>GGGSMEPGRGGTETVGKFEFSRKDLIGHGAFAVVFKGRHRAAHDLEVAVKCINKKNLAKSQTLLGKEIKILKELKHENIVALYDFQEMANSVYLVMEYCNGGDLADYLHAMRTLSEDTIRLFLQQIAGAMRLLHSKGIIHRDLKPQNILLSNPAGRRANPNSIRVKIADFGFARYLQSNMMAATLCGSPMYMAPEVIMSQHYDGKADLWSIGTIVYQCLTGKAPFQASSPQDLRLFYEKNKTLVPTIPRETSAPLRQLLLALLQRNHKDRMDFDEFFHHP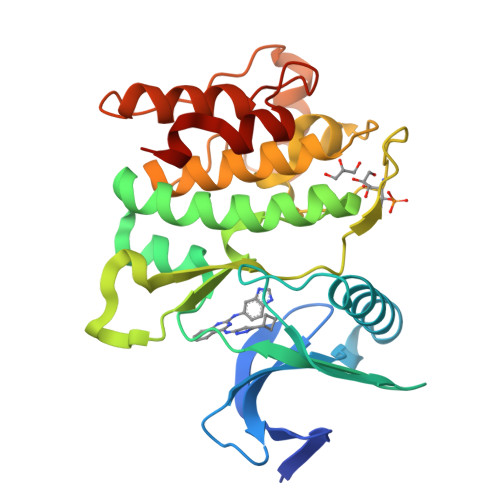FLDASPS[4x]Flavodoxins are electron transfer proteins that participate in a variety of reactions in prokaryotes and in some unicellular algae. The identification of flavodoxin as an essential protein for S. pneumoniae infectivity and the fact that flavodoxin is not present in humans open the possibility of using it as a target for the development of novel and specific antimicrobials against S. pneumoniae. According to its gene sequence translation, it contains 147 residues and very likely belongs to the so-called short-chain flavodoxins characterized by the lack of a 20-residue loop that, in the long-chain flavodoxins, appears intercalated in the fifth β-strand. Either structure shows the archetypical α/β sandwich flavodoxin fold (5 α-helices that pack against a five-stranded β-sheet with a 21345 topology, forming an α/β/α sandwich).

To understand the molecular basis of the interaction of the FMN cofactor with the protein moiety and to provide a structural frame for the identification and characterization of SpFld inhibitors, we have solved the crystal structures of the SpFld in the apo form and in complex with FMN, at 2.18 and 1.69 Å, respectively. Overall, the holo (note that the holo form contains selenomethionine (SeMet) residues) and apo SpFld structures are similar with an r.m.s.d of 0.8 Å. The main differences between the two structures are traced to two of the three FMN binding loops encompassing residues 10–14 (phosphate loop), 57–66 (50’ loop) and 92–100 (90’ loop), the latter two sandwiching the isoalloxazine moiety. Smaller changes are observed in the phosphate binding loop upon FMN binding because, in the different apoproteins studied, this loop always carries bound anions: a phosphate anion in Sp apoflavodoxin, a chloride anion in Helicobacter pylori, or a sulfate anion in Anabaena. Accommodation of the FMN into the Sp apoprotein takes place with changes in the dihedral angles of several residues of the isoalloxazine binding loops. In the 57–66 loop, the main changes are observed in residues G60, D61, G62 and E63, while in the 92–100 loop they occur in residues D92, Y95 and D96. No significant changes are noticed in the FMN phosphate binding loop, possibly reflecting that the conformation adopted by this loop in the apoprotein is highly influenced by the phosphate anion bound, which mimics the equivalent moiety in the FMN of the holoprotein. As previously reported for the apo/holo flavodoxin pairs in Anabaena PCC7119 and H. pylori, the entrance of the FMN cofactor makes the two isoalloxazine binding loops to move apart. In this reorganization, existing interactions between the two loops in the apoform (Y95/G60 and E97/G62) are broken and the protein expands: the holoprotein surface area is 7745 Å compared to 7135 Å for the apoprotein.

> GMALAKIVFASMTGNTEEIADIVADKLRDLGLDVDVDECTTVDASDFLEADIAIVATYTYGDGELPDEMMDFYEDLADLNLNGKIYGVVGSGDTFYDEFCKAVDDFDRVFVSTGAEKGSECVKVDLSAEEEDIERLEQFAEELAAKVGA>[2x]MRVPEKYSTLPAEDRSVHIVNICAIEDLGYLPSEGTLLNSLSVDPDAECKYGLYFRDGKRKVDYILVYHHKRASGSRTLARRGLQNDMVLGTRSVRQDQPLPGKGSPVDAGS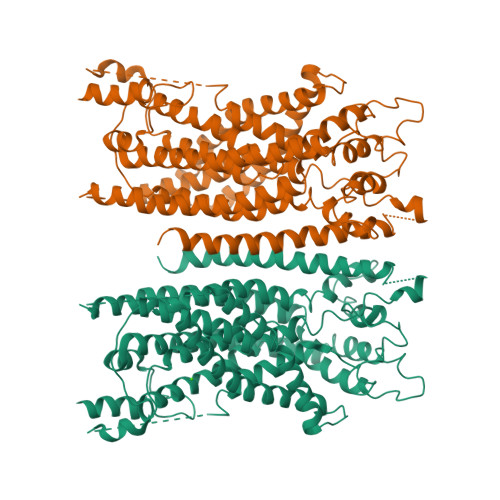PEVPMDYHEDDKRFRREEYEGNLLEAGLELENDEDTKIHGVGFVKIHAPWHVLCREAEFLKLKMPTKKVYHISETRGLLKTINSVLQKITDPIQPKVAEHRPQTTKRLSYPFSREKQHLFDLTDRDSFFDSKTRSTIVYEILKRTTCTKAKYSMGITSLLANGVYSAAYPLHDGDYEGDNVEFNDRKLLYEEWASYGVFYKYQPIDLVRKYFGEKVGLYFAWLGAYTQMLIPASIVGVIVFLYGCATVDENIPSMEMCDQRYNITMCPLCDKTCSYWKMSSACATARASHLFDNPATVFFSVFMALWAATFMEHWKRKQMRLNYRWDLTGFEEEEDHPRAEYEARVLEKSLRKESRNKETDKVKLTWRDRFPAYFTNLVSIIFMIAVTFAIVLGVIIYRISTAAALAMNSSPSVRSNIRVTVTATAVIINLVVIILLDEVYGCIARWLTKIEVPKTEKSFEERLTFKAFLLKFVNSYTPIFYVAFFKGRFVGRPGDYVYIFRSFRMEECAPGGCLMELCIQLSIIMLGKQLIQNNLFEIGIPKMKKFIRYLKLRRQSPSDREEYVKRKQRYEVDFNLEPFAGLTPEYMEMIIQFGFVTLFVASFPLAPLFALLNNIIEIRLDAKKFVTELRRPVAIRAKDIGIWYNILRGVGKLAVIINAFVISFTSDFIPRLVYLYMYSQNGTMHGFVNHTLSSFNVSDFQNGTAPNDPLDLGYEVQICRYKDYREPPWSEHKYDISKDFWAVLAARLAFVIVFQNLVMFMSDFVDWVIPDIPKDISQQIHKEKVLMVELSNSLEVLFQ>VGALAVVVW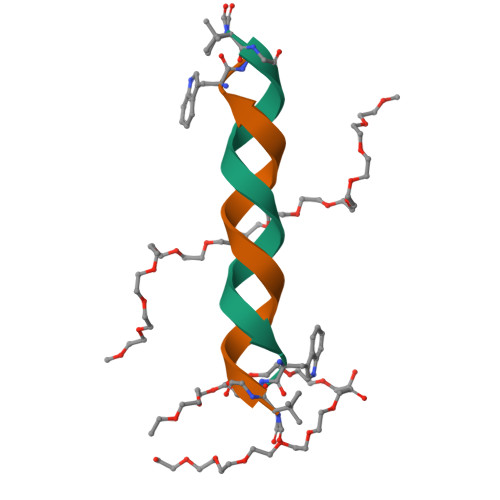LWLWLWX[6x]>[2x]GSHMELTPDQQTLLHFIMDSYNKQRMPQEITNKILK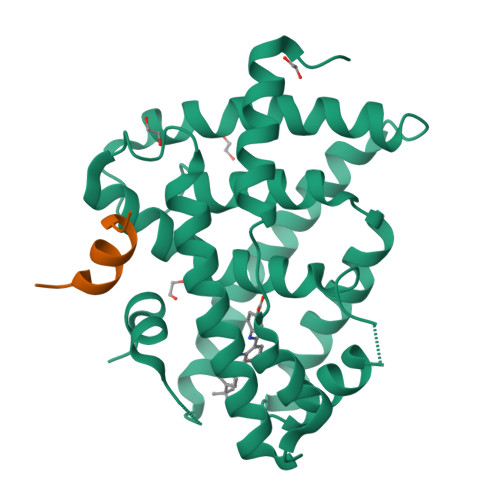EEFSAEENFLILTEMATNHVQVLVEFTKKLPGFQTLDHEDQIALLKGSAVEAMFLRSAEIFNKKLPSGHSDLLEERIRNSGISDEYITPMFSFYKSIGELKMTQEEYALLTAIVILSPDRQYIKDREAVEKLQEPLLDVLQKLCKIHQPENPQHFACLLGRLTELRTFNHHHAEMLMSWRVNDHKFTPLLCEIWDVQ;>[2x]KENALLRYLLDKD> MRKLYLFLFLTLISPISISIFHAQCTGATVESLTNPGPYTVATLSEADGVRNGPKYAGSTIYYPTNATPPYASIAIVPGFTAAPSSVQEWGPFYASHGIVAIIIGTNSLYDQPEARALALLDALETIKQENGRATSPLIGKLDVTKLAVSGWSMGGGGAQRAAVLDNTISAVVALCPYLTSPQLNHTVPVLIFSGQSDPTAPPSQHANVHYNTTPGTTNKLLFEVKNGNHSVANSPTGGGGAVGKLALSWLKIYLEKNDCYCSVLATAIVNSTTVSSKISQSYQCNNALGVVDSKTRFNLYPNPTKDFVQVNVRE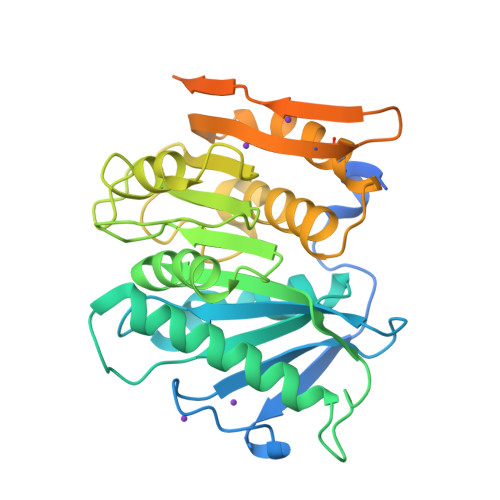MASYQLSSSTGQIVLKGIVTSSKNQIDLSKLPAGVYYLQINGETIKVIKKQ>GPLGSEFLWIEGIPFPTVYYSQEIIREVRDRFVVRDEDTIIVTYPKSGTHWLNEIVCLILTKGDPTWVQSTIANERTPWIEFENNYRILNSKEGPRLMASLLPIQLFPKS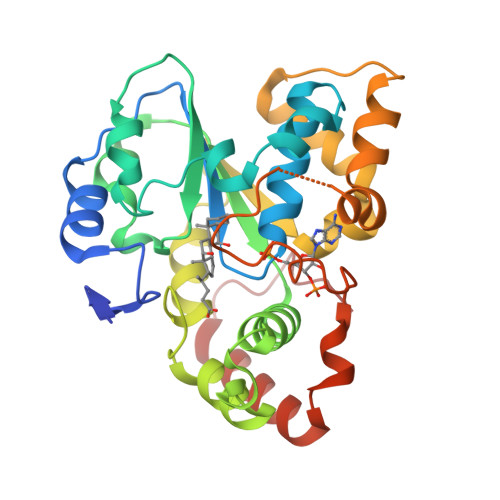FFSSKAKVIYLIRNPRDVLVSGYHYFNALKQGKEQVPWKIYFENFLQGKSYFGSWFEHACGWISLRKRENILVLSYEQLKKDTRNTIKKICEFLGENLESGELELVLKNISFQIMKERMISQSCLSNIEKHEFIMRKGITGDWKNHFTVAQAEAFDKAFQEKAADFPQELFSWE[2x]>[4x]VTAFLGERVTLTSYWRRVSLGPEIEVSWFKLGPGEEQVLIGRMHHDVIFIEWPFRGFFDIHRSANTFFLVVTAANISHDGNYLCRMKLGETEVTKQEHLSVVKPLTLSVHSERSQFPDFSVLTVTCTVNAFPHPHVQWLMPEGVEPAPSAANGGVMKEKDGSLSVAVDLSLPKPWHLPVTCVGKN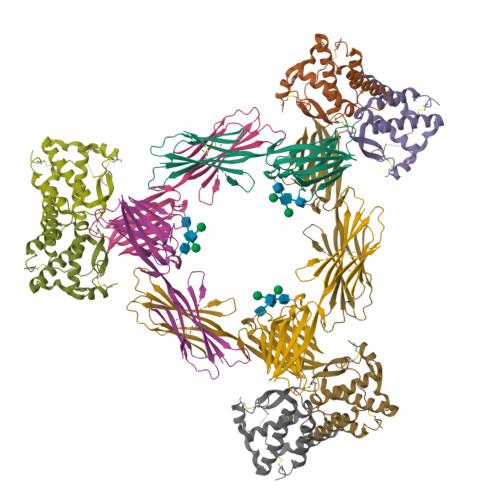DKEEAHGVYVSGYLSQKHHHHHH;>[4x]GSHMEEVSEYCSHMIGSGHLQSLQRLIDSQMETSCQITFEFVDQEQLKDPVCYLKKAFLLVQDIMEDTMRFRDNTPNAIAIVQLQELSLRLKSCFTKDYEEHDKACVRTFYETPLQLLEKVKNVFNETKNLLDKDWNIFSKNCNNSFAECSSQ The LRR-RKs HAESA (greek: to adhere to) and HAESA-LIKE 2 (HSL2) redundantly control floral abscission. A receptor protein called HAESA is found on the surface of the cells that surround a future break point on the plant. When its time to shed an organ, a hormone called IDA instructs HAESA to trigger the shedding process. The peptide hormone IDA binds to the HAESA LRR ectodomain.

A Hyp-modified dodecamer comprising the highly conserved PIP motif in IDA interacts with HAESA with 1:1 stoichiometry (N) and with a dissociation constant (Kd) of ~20 μM. We next determined crystal structures of the apo HAESA ectodomain and of a HAESA-IDA complex, at 1.74 and 1.86 Å resolution, respectively. IDA binds in a completely extended conformation along the inner surface of the HAESA ectodomain, covering LRRs 2–14. The central Hyp64IDA is buried in a specific pocket formed by HAESA LRRs 8–10, with its hydroxyl group establishing hydrogen bonds with the strictly conserved Glu266HAESA and with a water molecule, which in turn is coordinated by the main chain oxygens of Phe289HAESA and Ser311HAESA. The restricted size of the Hyp pocket suggests that IDA does not require arabinosylation of Hyp64IDA for activity in vivo, a modification that has been reported for Hyp residues in plant CLE peptide hormones. The C-terminal Arg-His-Asn motif in IDA maps to a cavity formed by HAESA LRRs 11–14. The COO- group of Asn69IDA is in direct contact with Arg407HAESA and Arg409HAESA and HAESA cannot bind a C-terminally extended IDA-SFVN peptide. This suggests that the conserved Asn69IDA may constitute the very C-terminus of the mature IDA peptide in planta and that active IDA is generated by proteolytic processing from a longer pre-protein. A N-terminal Pro-rich motif in IDA makes contacts with LRRs 2–6 of the receptor. The central Hyp residue in IDA is found buried in the HAESA peptide binding surface and thus this post-translational modification may regulate IDA bioactivity.

> GSSMGSLNQDATILRQAKLGLSDPAQSLSSWSDNNDVTPCKWLGVSCDATSNVVSVDLSSFMLVGPFPSILCHLPSLHSLSLYNNSINGSLSADDFDTCHNLISLDLSENLLVGSIPKSLPFNLPNLKFLEISGNNLSDTIPSSFGEFRKLESLNLAGNFLSGTIPASLGNVTTLKELKLAYNLFSPSQIPSQLGNLTELQVLWLAGCNLVGPIPPSLSRLTSLVNLDLTFNQLTGSIPSWITQLKTVEQIELFNNSFSGELPESMGNMTTLKRFDASMNKLTGKIPDNLNLLNLESLNLFENMLEGPLPESITRSKTLSELKLFNNRLTGVLPSQLGANSPLQYVDLSYNRFSGEIPANVCGEGKLEYLILIDNSFSGEISNNLGKCKSLTRVRLSNNKLSGQIPHGFWGLPRLSLLELSDNSFTGSIPKTIIGAKNLSNLRISKNRFSGSIPNEIGSLNGIIEISGAENDFSGEIPESLVKLKQLSRLDLSKNQLSGEIPRELRGWKNLNELNLANNHLSGEIPKEVGILPVLNYLDLSSNQFSGEIPLELQNLKLNVLNLSYNHLSGKIPPLYANKIYAHDFIGNPGLCVDLDGLCRKITRSKLEGSENLYFQ;> PIPPSAPSKRHN7-[2-[2,4-bis(fluoranyl)phenoxy]-5-(2-oxidanylpropan-2-yl)phenyl]-2-[4-(2-hydroxyethyloxy)-3,5-dimethyl-phenyl]-5-methyl-furo[3,2-c]pyridin-4-one | C33 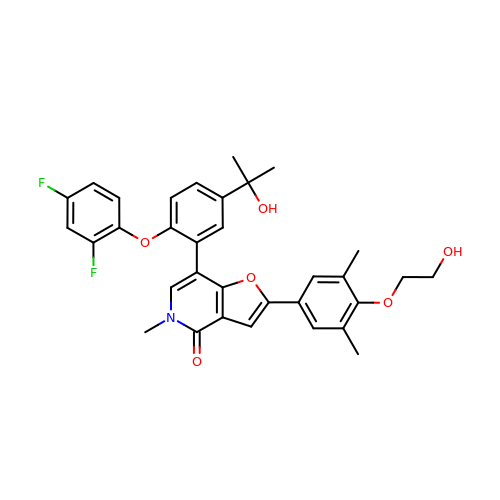H31 F2 N O6 | MCDGNYQOWDNEJL-UHFFFAOYSA-N>GSMVLNGYWGYQEFLDEFPEQRNLTNALSEAVRAQPVPLSKPTQRPIKISVVYPGQQVSDYW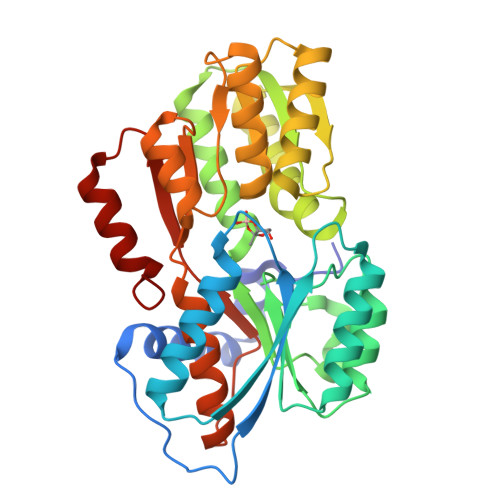VRNIASFEKRLYKLNINYQLNQVFTRPNADIKQQSLSLMEALKSKSDYLIFTLDTTRHRKFVEHVLDSTNTKLILQNITTPVREWDKHQPFLYVGFDHAEGSRELATEFGKFFPKHTYYSVLYFSEGYISDVRGDTFIHQVNRDNNFELQSAYYTKATKQSGYDAAKASLAKHPDVDFIYACSTDVALGAVDALAELGREDIMINGWGGGSAELDAIQKGDLDITVMRMNDDTGIAMAEAIKWDLEDKPVPTVYSGDFEIVTKADSPERIEALKKRAFRYSDN[2x]>[8x]ETLVRPKPLLLKLLKSVGAQKDTYTMKEVLFYLGQYIMTKRLYDEKQQHIVYCSNDLL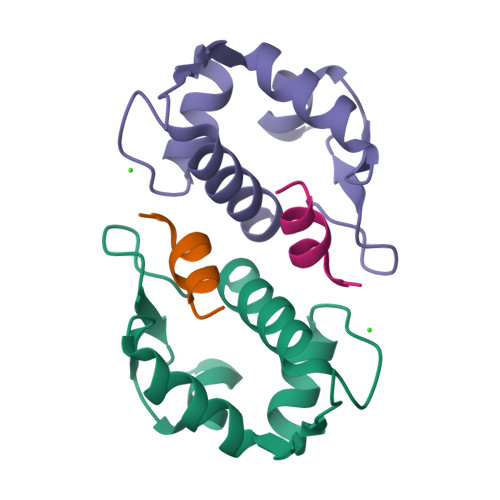GDLFGVPSFSVKEHRKIYTMIYRNLVV;>TSFAEYWALLSP[8x]>[2x]DYKDDDDEGPAKKVLTLEGDLVLGGLFPVHQKGGPAEDCGPVNEHRGIQRLEAMLFALDRINRDPHLLPGVRLGAHILDSCSKDTHALEQALDFVRASLSRGADGSRHICPDGSYATHGDAPTAITGVIGGSYSDVSIQVANLLR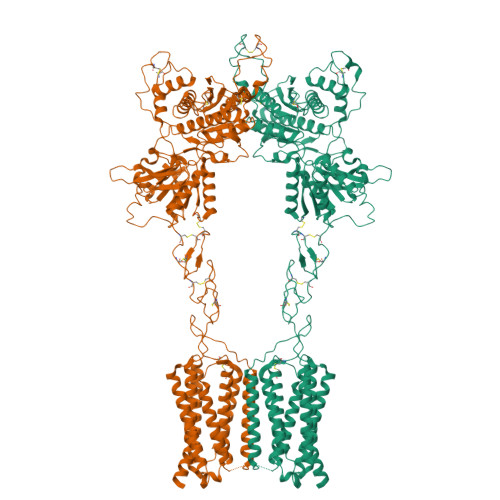LFQIPQISYASTSAKLSDKSRYDYFARTVPPDFFQAKAMAEILRFFNWTYVSTVASEGDYGETGIEAFELEARARNICVATSEKVGRAMSRAAFEGVVRALLQKPSARVAVLFTRSEDARELLAASQRLNASFTWVASDGWGALESVVAGSEGAAEGAITIELASYPISDFASYFQSLDPWNNSRNPWFREFWEQRFRCSFRQRDCAAHSLRAVPFEQESKIMFVVNAVYAMAHALHNMHRALCPNTTRLCDAMRPVNGRRLYKDFVLNVKFDAPFRPADTHNEVRFDRFGDGIGRYNIFTYLRAGSGRYRYQKVGYWAEGLTLDTSLIPWASPSAGPLPASRCSEPCLQNEVKSVQPGEVCCWLCIPCQPYEYRLDEFTCADCGLGYWPNASLTGCFELPQEYIRWGDAWAVGPVTIACLGALATLFVLGVFVRHNATPVVKASGRELCYILLGGVFLCYCMTFIFIAKPSTAVCTLRRLGLGTAFSVCYSALLTKTYRIARIFGGAREGAQRPRFISPASQVAICLALISGQLLIVVAWLVVEAPGTGKETAPERREVVTLRCNHRDASMLGSLAYNVLLIALCTLYAFKTRKCPENFNEAKFIGFTMYTTCIIWLAFLPIFYVTSSDYRVQTTTMCVSVSLSGSVVLGCLFAPKLYIILFQPQKNVEFLEVLFQ>SREFDFFTYETPKVIVVKSWTIGIINRVVQLLIISYFVGWVFLHEKAYQVRDTAIESSVVTKVKGSGLYANRVMDVSDYVTPPQGTSVFVIITKMIVTENQMQGFCPESEEKYRCVSDSQCGPERLPGGGILTGRCVNYSSVLRTCEIQGWCPTEVDTVETPIMMEAENFTIFIKNSIRFPLFNFEKGNLLPNLTARDMKTCRFHPDKDPFCPILRVGDVVKFAGQDFAKLARTGGVLGIKIGWVCDLDKAWDQCIPKYSFTRLDSVSEKSSVSPGYNFRFAKYYKMENGSEYRTLLKAFGIRFDVLVYGNAGKFNIIPTIISSVAAFTSVGVGTVLCDIILLNFLKGADQYKAKKFEEVNE[3x]

P2X3 receptors are a family of trimeric cation channels that are activated by extracellular ATP. They play particularly important roles in sensory neurons where their activation is critical for gustatory and nociceptive responses (Barclay et al., 2002; Chen et al., 1995; Cook et al., 1997; Finger et al., 2005; Huang et al., 2011; North, 2003; North, 2004; Vandenbeuch et al., 2015), visceral reflexes and sensory hypersensitization. P2X3 homomeric receptors activate and desensitize on the millisecond timescale upon binding ATP but unbind ATP and recover from desensitization on the timescale of minutes. Although free-ATP is an agonist in laboratory conditions, P2X3 receptors are activated primarily by Ca2+-ATP and Mg2+-ATP under physiological conditions because ATP released from cells at micromolar concentrations would largely be in complex with Ca2+ and Mg2+, both of which are present in millimolar concentrations in extracellular physiological solutions.

We began by crystalizing the hP2X3 MFCslow construct in solutions containing ATP with either Mg2+ or Ca2+. We solved X-ray structures of the receptor with Mg2+-ATP or Ca2+-ATP bound at resolutions of 3.8 Å and 3.3 Å, respectively. The pores appear to be in an open-like conformation in both structures, similar to that observed in the structure of hP2X3 bound to free-ATP. Importantly, we observed strong residual electron densities around the ATP binding site in these structures. Considering that the crystallization conditions included either 50 mM Mg-acetate or 50 mM Ca-acetate with no other divalent cations, and that the electron densities are surrounded by acidic residues, we interpreted the densities as Mg2+ and Ca2+ ions, respectively. In both structures, the divalent ions are detected at the edge of the ATP binding pocket, simultaneously interacting with D158 on the receptor and with the γ-phosphate of ATP; E156 is also positioned nearby and appears to be involved in coordinating the ion. A survey of the Protein Data Bank (PDB) reveals that the geometry of the Mg2+-ATP and Ca2+-ATP complexes observed in our structures is highly unusual. By contrast, the presence of 1 mM Mg2+ slowed deactivation by ~8-fold, while 1 mM Ca2+ slowed deactivation by ~ 4 fold, suggesting that both ions slow ATP dissociation. Although both Mg2+ and Ca2+ ions slow hP2X3 slow deactivation, the effect of Ca2+ is more modest when compared to Mg2+, suggesting that Ca2+ might compete with Mg2+ to hasten unbinding under physiological conditions. Interestingly, the influence of Ca2+ on stabilizing ATP on the receptor and slowing recovery from desensitization is less pronounced than for Mg2+, which could explain why Ca2+ can facilitate activation of P2X3 receptors in physiological solutions containing Mg2+ in response to repeated applications of ATP.>[4x]ADD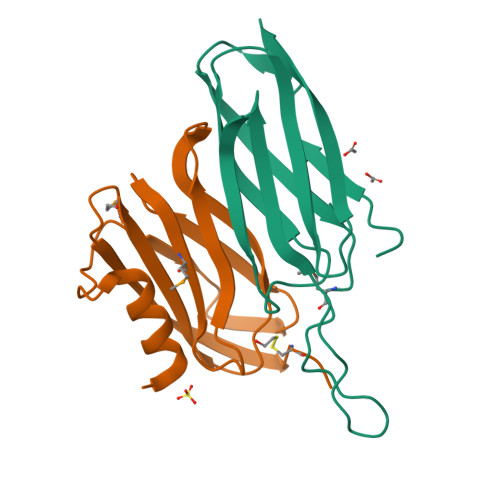AKPRVKVPSSAKAGETVTVKALISHKMESGQRKDADGKLIPRSIINRFTCELNGVNVVDVAIDPAVSTNPYFEFDAKVDAAGEFKFTWYDDDGSVYEDVKPIAVA;>[4x]HGSSTVDELTAAFTGGAATGEGGLTLTAPEIAENGNTVPIEVKAPGAVAIMLLAAGNPEPAVATFNFGPAAADQRAATRIRLAQTQDVIALAKMADGSVVKAQTTVKVTIGGCGG> MGSLLALLALLLLWGAVAEGPAKKVLTLEGDLVLGGLFPVHQKGGPAEDCGPVNEHRGIQRLEAMLFALDRINRDPHLLPGVRLGAHILDSCSKDTHALEQALDFVRASLSRGADGSRHICPDGSYATHGDAPTAITGVIGGSYSDVSIQVANLLRLFQIPQISYASTSAKLSDKSRYDYFARTVPPDFFQAKAMAEILRFFNWTYVSTVASEGDYGETGIEAFELEARARNICVATSEKVGRAMSRAAFEGVVRALLQKPSARVAVLFTRSEDARELLAASQRLNASFTWVASDGWGALESVVAGSEGAAEGAITIELASYPISDFASYFQSLDPWNNSRNPWFREFWEQRFRCSFRQRDCAAHSLRAVPFEQESKIMFVVNAVYAMAHALHNMHRALCPNTTRLCDAMRPVNGRRLYKDFVLNVKFDAPFRPADTHNEVRFDRFGDGIGRYNIFTYLRAGSGRYRYQKVGYWAEGLTLDTSLIPWASPSAGPLPASRCSEPCLQNEVKSVQPGEVCCWLCIPCQPYEYRLDEFTCADCGLGYWPNASLTGCFELP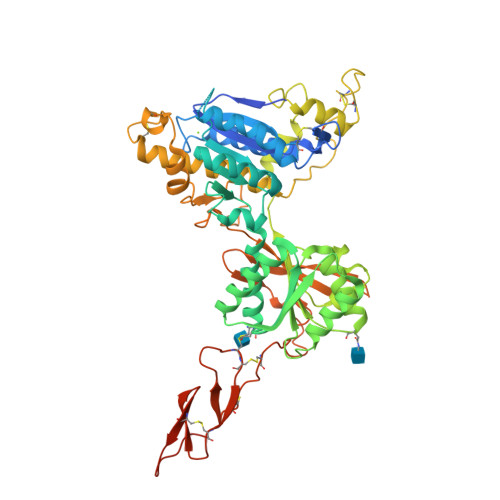QEYIREGHHHHHH> MKTFIFLALLGAAVAFPVDDDDKIVGGYTCGANTVPYQVSLNSGYHFCGGSLINSQWVVSAAHCYKSGIQVRLGEDNINVVEGNEQFISAS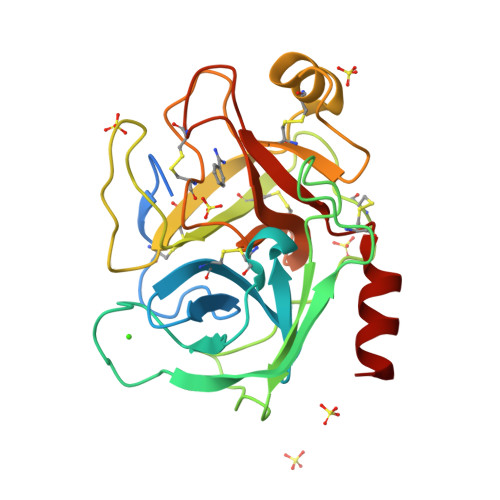KSIVHPSYNSNTLNNDIMLIKLKSAASLNSRVASISLPTSCASAGTQCLISGWGNTKSSGTSYPDVLKCLKAPILSDSSCKSAYPGQITSNMFCAGYLEGGKDSCQGDSGGPVVCSGKLQGIVSWGSGCAQKNKPGVYTKVCNYVSWIKQTIASN>[2x]GMSKLSLIQQLKQQKLS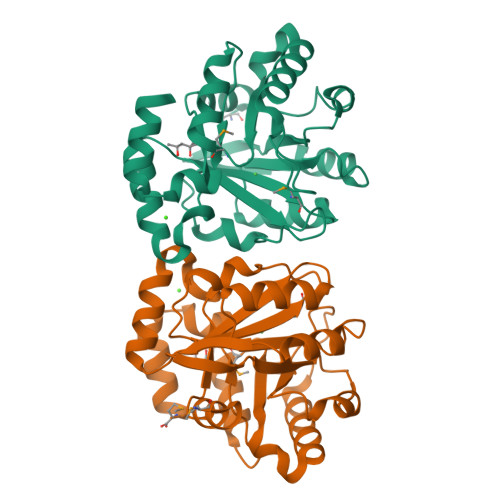VGILSANWLQLNEEVTTLLENQINVLHFDIADGQFSSLFTVGAIGIKYFPTHCFKDVHLMVRNQLEVAKAVVANGANLVTLQLEQYHDFALTIEWLAKQKTTYANQVYPVLIGACLCPETPISELEPYLDQIDVIQLLTLDPRNGTKYPSELILDRVIQVEKRLGNRRVEKLINIDGSMTLELAKYFKQGTHQIDWLVSGSALFSGELKTNLKVWKSSIM>[2x]GSGSHVTLPFYPKSPQSKDLIKEAILDNDFMKNLELSQIQEI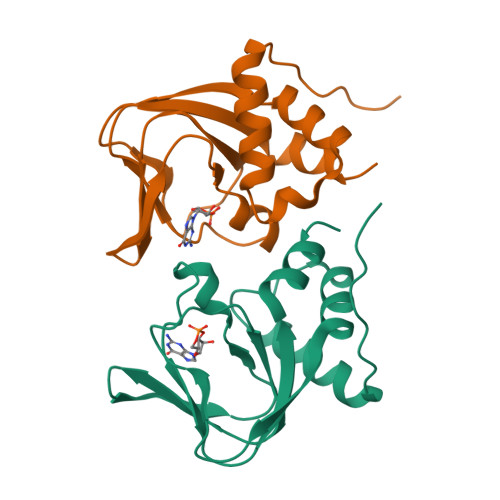VDCMYPVEYGKDSCIIKEGDVGSLVYVMEDGKVEVTKEGVKLCTMGPGKVFGELAILYNCTRTATVKTLVNVKLWAIDRQCFQTIMMRTGLIKHTEY5-chloro-7-(2-(2-(2,4-dioxo-3,4-dihydropyrimidin-1(2H)-yl)ethoxy)phenoxy)-8-methyl-2-naphthonitrile 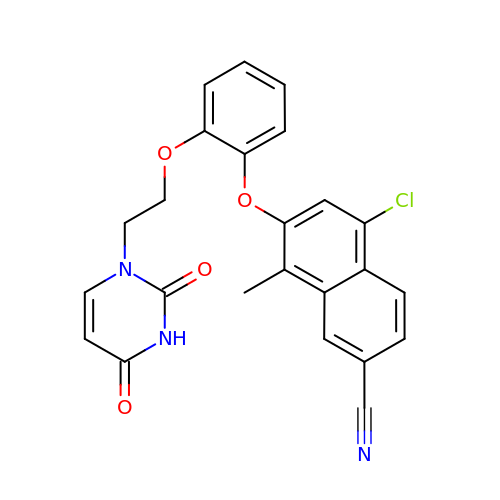| C24 H18 Cl N3 O4 | KFUNYNPQHKSQRQ-UHFFFAOYSA-N> NE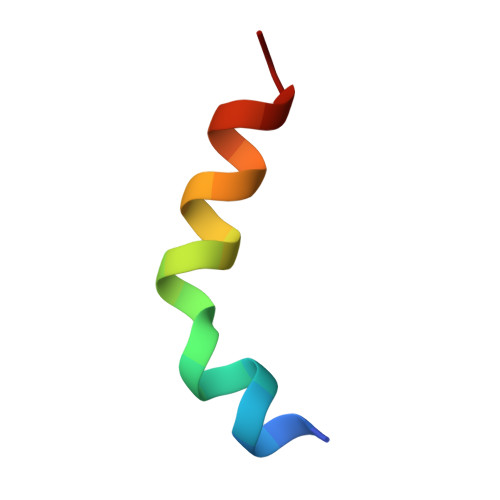DIDQMFSTLLGEMDLLTQS> TTCCPSIVARSNFNVCRLPGTPEAICATYTGCI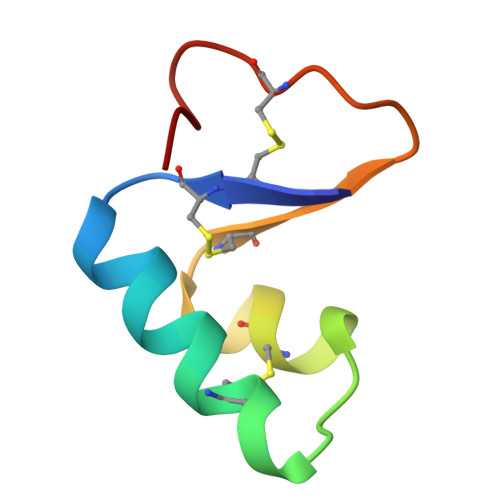IIPGATCPGDYAN> MTEKEEKEDLQAQDKEEQQIKADTKVISVQEFEEYMRFKEQANSKSKETSRDLSINERITKELAEVEERERIEKQLLLEAERINEIDTLAKAHLSNHFNKEVLLAKGYTLKDIMQAQRRELVRKFVPIEQIKAIAKVSDISHI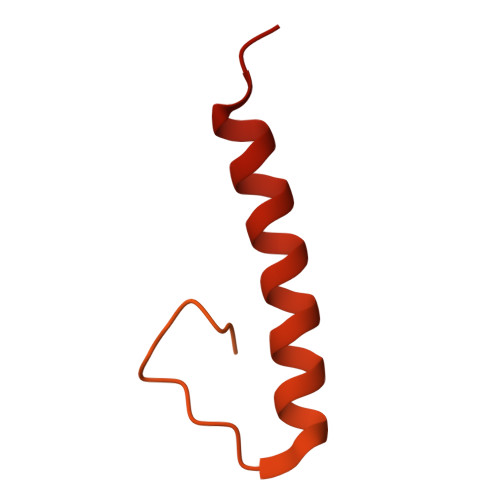DGEILEQLVSLAKVNIKLRKNASSSSSSVDSIKGNIAIKSEERASLLDSNFVPINFTEFVQAISNTYKQRRIQFYENLKRHKRTSIA> MVAENQPGHIDQIKQTNAGAVYRLIDQLGPVSRIDLSRLAQLAPASITKIVREMLEAHLVQELEIKEAGNRGRPAVGLVVETEAWHYLSLRISRGEIFLALRDLSSKLVVEESQELALKDDSPLLDRIISHIDQFFIRHQKKLERLTSIAITLPGIIDTENGIVHRMPFYEDVKEMPLGEALEQHTGVPVYIQHDISAWTMAEALFGASRGARDVIQVVIDHNVGAGVITDGHLLHAGSSSLVEIGHTQVDPYGKRCYCGNHGCLETIASVDSILELAQLRLNQSMSSMLHGQPLTVDSLCQAALRGDLLAKDIITGVGAHVGRILAIMVNLFNPQKILIGSPLSKAADILFPVISDSIRQQALPAYSQHISVESTQFSNQGTMAGAALVKDAMYNG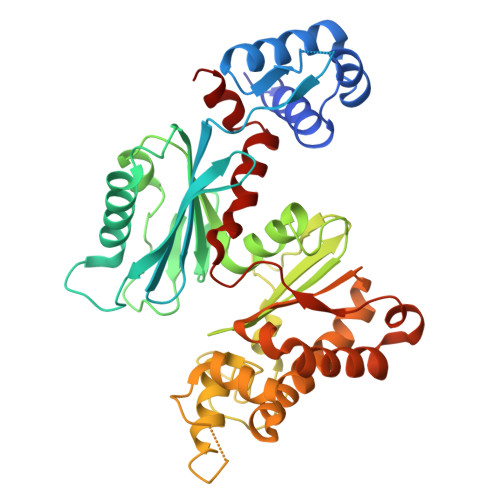SLLIRLLQG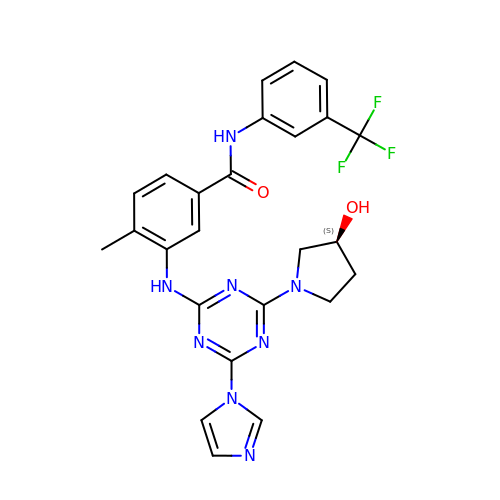3-[[4-imidazol-1-yl-6-[(3~{S})-3-oxidanylpyrrolidin-1-yl]-1,3,5-triazin-2-yl]amino]-4-methyl-~{N}-[3-(trifluoromethyl)phenyl]benzamide | C25 H23 F3 N8 O2 | IOGRLXUUAIVKHX-IBGZPJMESA-N11,15-dimethyl-6-(4-methylpiperazin-1-yl)-8-oxa-2,11,15,19,21,23-hexazatetracyclo[15.6.1.13,7.020,24]pentacosa-1(23),3(25),4,6,17,20(24),21-heptaen-10-one 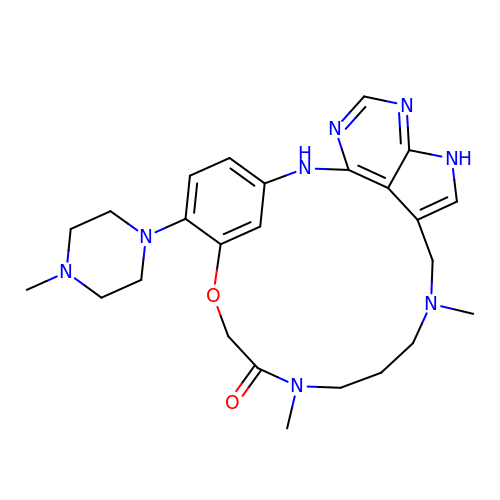| C25 H34 N8 O2 | SOJXCMRVYOLJEH-UHFFFAOYSA-N>MLKFMLDTNICIFTIKNKPASVRERFNLNQGKMCISSVTLMELIYGAEKSQMPERNLAVIEGFVSRIDVLDYDAAAATHTGQIRAELARQGRPVGPFDQMIAGHARSRGLIIVTNNTREFERVGGLRTEDWS[4x];>[4x]MHHHHHHETTVFLSNRSQAVRLPKAVALPENVKRVEVIAVGRTRIITPAGETWDEWFDGHSVSTDFMDNREQPGMQERESF

Toxin–antitoxin (TA) loci are widespread in prokaryotes and code for an active “toxin” molecule, typically, a translational regulator, and an “antitoxin” that forms a tight complex with the toxin and thus inhibits it. In the largest TA family, vapBC, the VapC toxin contains a PilT N-terminal (PIN) domain, which is a compact ribonuclease domain consisting of an αβ-fold harboring four highly conserved acidic residues required for catalysis. Recently, it was found that VapC (MvpT) from the Gram-negative pathogen Shigella flexneri 2a virulence plasmid pMYSH6000 functions by specifically cleaving initiator tRNAfMet in the anticodon region, thus globally down-regulating translation. In order to understand the activity, mode of inhibition, and DNA-binding properties of the VapBC family, we have determined the crystal structure of the VapBC complex from S. flexneri.

The asymmetric unit contains four copies of both VapB and VapC, for which the VapC structures are complete (residues 1–132), while the VapB structures cover residues 2–67 of the complete sequence (1–75). S. flexneri VapC contains a typical PIN domain structure consisting of a small and central five-stranded β-sheet (β1–β5) surrounded by seven α-helices, denoted α1 through α7 (blue). VapB has an N-terminal domain consisting of four β-strands (residues 1–45), which dimerizes with a neighboring VapB to form a complete DNA-binding domain, and an extended C-terminal tail (residues 46–67) that wraps around VapC (orange). In the crystal, the four copies of VapBC in the asymmetric unit form a large and globular VapB4C4 hetero-octameric assembly, consisting of two VapB2C2 complexes related to each other by a dyad axis (Fig. 1b, top view; the dyad is indicated by the black lens shape at the center). The structure reveals a compact hetero-octameric assembly with two unique DNA-binding domains of the SpoVT/AbrB type that have not been previously observed in VapBC complexes. Firstly, four aromatic residues in VapB (Trp47, Trp50, Phe51, and Phe60) point into the hydrophobic interface between helices α1, α2, α3, and α4 of VapC where they interact tightly with the hydrophobic core of the protein. Secondly, near the C-terminus of VapB, the side chains of Arg64 and Gln66 of VapB point directly into the active site of VapC, where they make close, charged interactions to the conserved acidic active residues Asp7, Glu42, and Asp98. Mutant studies implicate metal ion 1 (right) directly in the cleavage mechanism, whereas metal ion 2 (left) is thought to stabilize the conformation of the active site and enhance substrate binding. Both ions are present in the FEN-1 structure, and comparison to VapC reveals that the positively charged guadinium group of Arg64 in VapB appears to take up the position of metal ion 1, while Gln66 may substitute metal ion.> MQQTTSTKDSSKGTTYYVSSEHGSDDNAGTSQKSPWKTLNKVNEIASDLEPGDSVLLEYGSEFNDQWLHIHDTAGTPDAPITISAYGDEAEGKPLIASNGVEGSQWYQDYRANVGNHKTRGTVSTTLLLKDVSYITVSNLEITNDDESVYDPIDTWQWTDTADADGTSLDRSADRMDRTGVAGIAENGSTMSHVTLDNLNIHDVDGNLYNKHMANGGIYFMAHLPKERTSAADDAWLKEHVSRFDHITIRNSTVKDVDRWGIAVGYTAYLNYIDKSSRWQNDFDYGDGTIDDDLIAKYGATNVLIENNTIIGAGGDAITTMYCDRPVIQHNVGDRVSKHINSVDYTANVLNNTGNAGVGYGRVAAGIWPWRCKDPVFQYNEVYSNLNADHGNGDGQAWDADYGDGTLYQYNYSYGNSFASL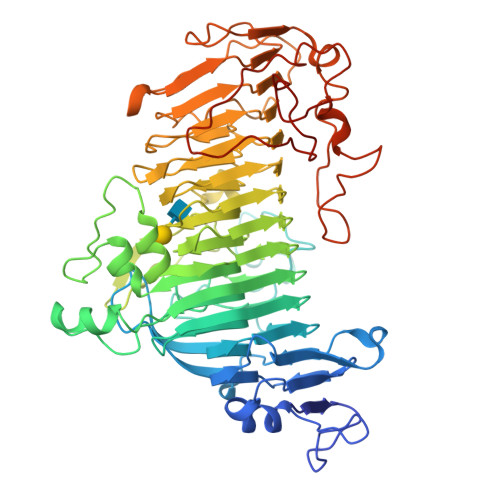MICNWKAVNTTFRYNISQNDKRGVFDLPSNGPGNHIYNNTVYVDADSRVLTTRSNSQAQFENNIFINATDEKKTEEWNIGGYYGGQVYDNNLYVNYANTPASDANAIVADDVADVLEDAGSAPTAAQASGAEYSRKGSTTVFDGYKPTTNSPAINAGKVVSDLNDYAVEHDFFGNTIKGKPDLGAVESAAALEHHHHHH>ETGKDIVKILTASTTVTKTGPPPISAECPHNMVVLFGFVVKQNFWDHTNKLQSYEMEICESGASSCTSKQGNTNKYDVSYTYIECGPQALPFTEQVVSVSGTTYNSVKCPNDYSVLFG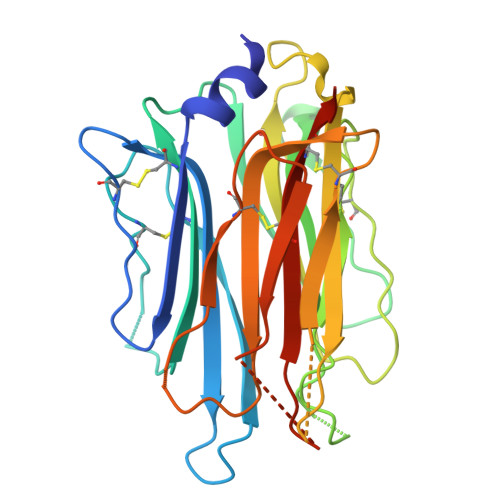FGMATSSGRHQSALYSYFTPCRPGLKSCSLNMNEHDDKSYIYLVCVDATIWTGLNALSMIAKDDLHSAVNRYQQFNDGELVVTCPSEGTILTGFYGETHTSSPYVTVPFGKCAKSLKACSVHGSGQAIGIHNYRTLFTVALCKNNKTHHHHHH[2x]>GSPKLPRGLRFGADNEILNDFQELWFPDLFIESSDTHPWYTLKGRVLNAHLDDRLPNVGGRQVRRTPHRVTVPIASSGLRPVTTVQYDPAALSFLLNARVDWDFGNGDSANLVINDFLFRTFAPKEFDFSNSLVPRYTQAFSAFNAKYGTMIGEGLETIKYLGLLLRRLREGYRAVKRGDLRALRRVIQSYHNGKWKPATAGNLWLEFRYGLMPLFYDIRDVMLDWQNRHDKIQRLLRFSVGHGEDYVVEFDNLYPAVAYFK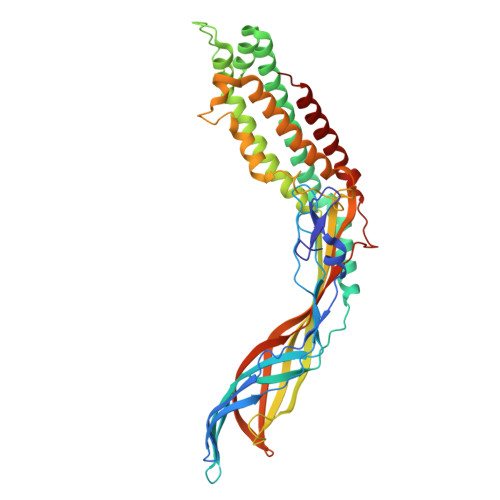LKGEITLERRHRHGISYANREGYAVFDNGSLRPVSDWKELATAFINPHEVAWELTPYSFVVDWFLNVGDILAQQGQLYHNIDIVDGFDRRDIRLKSFTIKGERNGRPVNVSASLSAVDLFYSRLHTSNLPFATLDLDTTFSSFKHVLDSIFLLTQRVKR[4x]> MPNNESIVVEIVKLKNFHVYRGVSPIGVKDYQVGQKIVKSTSTDEHGNPVGLGNYDPHWQGLYAAEHLHHAASYAVDNNSGVPGGLFKIKLPEDVRFVRYENKDAAQAITPGRLYRALREEGLIKLTTAKELNETHFNSNQNFLTNELGKEKIILIDTDEFESFTDINGMKIPRLEFIIPWNIATEQVQVSEEVKVWYKGRDFSSLNAKERLELMMKLRGPYENDLTSYEAKFKDLIICRSASYYSSGSSCLDWEKIKTESQRIVKQIIEEHPELQSHSKNAVTDKEKLQKIYNDYAPKIDKLSSLKEGVSRATTALNIASWAAGLAETFSNKNADGLDKAAAVTAIIPGLGQAVGIANGIEKHDGEAIAINSIALSALVVAQAIPIVGEIADVVGAGLILAGGLAQLIQSVSPDTPPHVEPPHFYPQTSNHVTVGWLNQKIDEMIHAWYPHEGYRSHHFVIKIANDAPENTTMPITEIMAKLGSQTKQLDLVPERVWVYQNNNVITCTKQTVSLKTDRFAVIRPLFPTMLTKSRPIVVRMAYITGENSCTTDANPTCFPENPAIAVRVTPLPSNNECEWDHTPLHPSYQNGDKADFVRLGYRIGV

DT homologs from Streptomyces albireticuli (17% identity to DT) and Seinonella peptonophila (20% identity to DT), despite showing no toxicity toward human cells, display significant structural similarities to DT sharing both the overall Y-shaped architecture of DT as well as the individual folds of each domain. Moreover, each of the individual domains preserve their respective folds: the central split β-sheet motif in the catalytic domain characteristic of the ADP-ribosyl transferase (ADPRT) superfamily; the three-layered α-helical translocation domain; and, the Ig-like jelly-roll fold in the receptor-binding domain. Additionally, both DT homologs maintain the pinched disulfide loop at the junction between the C- and T-domains. Given these structural similarities, and for purposes of clarity and simplicity, we refer to these two DT homologs hereafter as Albireti Toxin (AT) and Peptono Toxin (PT). By striking contrast, we found that AT and PT do not display any measurable toxicity on Vero cells even at µM concentrations.

As crystals of the DT homolog from S. peptonophila were grown in a condition containing potassium iodide, a 2.2 Å dataset was collected with native protein crystals at a wavelength of 2.0 Å to maximize the anomalous signal from iodide. The structure was subsequently solved using iodide-SAD phasing. Whereas the homolog from S. albireticuli (S.a) displays a Tm comparable to DT (46.5 °C cf. 48.25 °C), the homolog from S. peptonophila (S.p) is significantly more thermostable (Tm = 59.5 °C). Of note, however, AT and PT contain both Cys residues (C217/C231 and C239/C251, respectively) that bound this region, and the crystal structures confirm formation of the inter-fragment disulfide bonds. In ATR and PTR, the 16 amino acid insertion between β9 and β10 contributes to an ~25 amino acid “lid,” hinging at ATG550 and ATN576 (PTP571 and PTD596), that folds back over and occludes the presumed receptor binding surface. By contrast, in AT and PT, only Y54 and E148 are absolutely conserved: in both, an Arginine is seen in place of the H21 residue; and in AT an Asparagine is seen in place of Y65. The T domain of PT contains three His residues: H272, H276, and H364. Two of these residues are structurally equivalent with His residues in DT: PTH272 ↔ DTH223 and PTH364 ↔ DTH322. Rather than forming π-stacking interactions with a second His residue as in DT, PTH272 forms an edge-to-face π–π interaction with PTY296.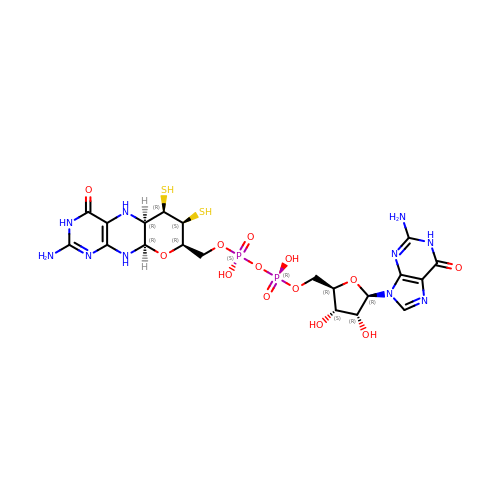GUANYLATE-O'-PHOSPHORIC ACID MONO-(2-AMINO-5,6-DIMERCAPTO-4-OXO-3,5,6,7,8A,9,10,10A-OCTAHYDRO-4H-8-OXA-1,3,9,10-TETRAAZA-ANTHRACEN-7-YLMETHYL) ESTER | C20 H28 N10 O13 P2 S2 | YDYCAANTTOPADF-JKOCJXFLSA-N>MNKPQTIYEKLGGENAMKAAVPLFFKKVLADERVKHFFKNTDMDHQTKQQTDFLTMLLGGPNHYKGKNMTEAHKGMNLQNLHFD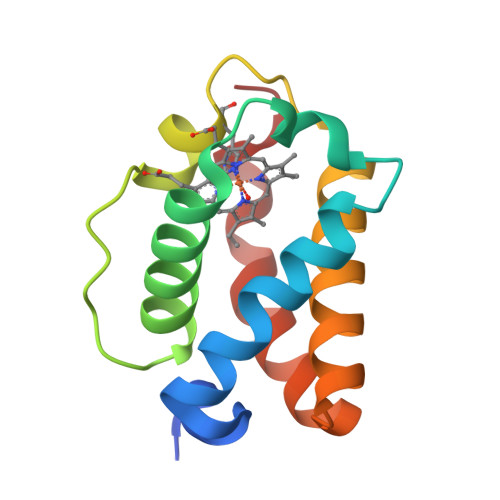AIIENLAATLKELGVTDAVINEAAKVIEHTRKDMLGK[2x]(S)-4'-hydroxy-3'-(6-methyl-2-oxo-3-(1H-pyrazol-4-yl)indolin-3-yl)-[1,1'-biphenyl]-2,4-dicarboxylic 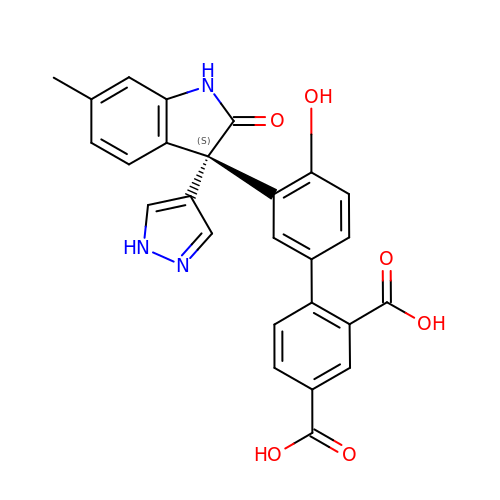acid | C26 H19 N3 O6 | QNQTUANCNUSMBX-AREMUKBSSA-N>MVLPDIKKGKDMINILPFEIISRNTKTLLITYISSVDITHEGMKKVLESLRSKQGIISEYLLDKLLDESLIDKDKGKEFLITTGVINKTKTSPLWVNSVIISDVPHLFSNAREQWKCDGVFVSHIIDIKDNNINVSDSTLIWLHLENYHSDIVKRIYSKFESNPGVAFIQSYYLKESFRIDGVYSPDLGTPCHFCHIERWLSREEKSFRRNEMSWANLLQLLKKYQMTLPALALGESERGFSYHLIKRRLQELTGTSLVKSHVDNFMSSVSADLITCILCKEPVIHWQACSCLER[2x];> MGHHHHHHMELKASEFGVVLSVDALKLSRQSPLGVGIGGGGGGGGGGSCGGQGG;> MSKHELSLVEVTHYTDPEVLAIVKDFHVRGNFASLPEFAERTFVSAVPLAHLEKFENKEVLFRPGFSSVINISSSHNFSRERLPSGINFCDKNKLSIRTIEKLLVNAFSSPDPGSVRRPYPSGGALYPIEVFLCRLSENTENWQAGTNVYHYLPLSQALEPVATCNTQSLYRSLSGGDSERLGKPHFALVYCIIFEKALFKYRYRGYRMALMETGSMYQNAVLVADQIGLKNRVWAGYTDSYVAKTMNLDQRTVAPLIVQFFGDVNDDKCLQ;> MINVYSNLMSAWPATMAMSPKLNRNMPTFSQIWDYERITPASAAGETLKSIQGAIGEYFERRHFFNEIVTGGQKTLYEMMPPSAAKAFTEAFFQISSLTRDEIITHKFKTVRAFNLFSLEQQEIPAVIIALDNITAADDLKFYPDRDTCGCSFHGSLNDAIEGSLCEFMERQSLLLYWLQGKANTEISSEIVTGINHIDEILLALRSEGD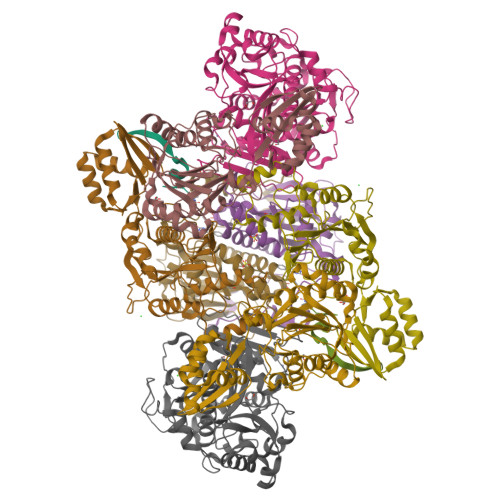IRIFDITLPGAPGHAVLTLYGTKNKISRIKYSTGLSYANSLKKALCKSVVELWQSYICLHNFLIGGYTDDDIIDSYQRHFMSCNKYESFTDLCENTVLLSDDVKLTLEENITSDTNLLNYLQQISDNIFVYYARERVSNSLVWYTKIVSPDFFLHMNNSGAININNKIYHTGDGIKVRESKMVPFP>TSLFTTADHYHTPLGPDGTPHAFFEALRDEAETTPIGWSEAYGGHWVVAGYKEIQAVIQNTKAFSNKGVTFPRYETGEFELMMAGQDDPVHKKYRQLVAKPFSPEATDLFTEQLRQSTNDLIDARIELGEGDAATWLANEIPARLTAILLGLPPEDGDTYRRWVWAITHVENPEEGAEIFAELVAHARTLIAERRTNPGNDIMSRVIMSKIDGESLSEDDLIGFFTILLLGGIDNTARFLSSVFWRLAWDIELRRRLIAHPELIPNAV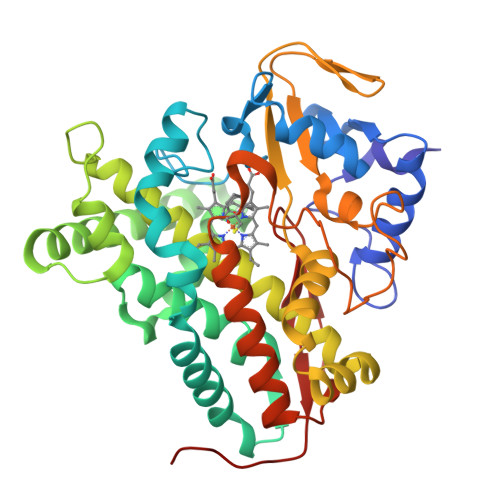DELLRFYGPAMVGRLVTQEVTVGDITMKPGQTAMLWFPIASRDRSAFDSPDNIVIERTPNRHLSLGHGIHRCLGAHLIRVEARVAITEFLKRIPEFSLDPNKECEWLMGQVAGMLHVPIIFPKGKRLSE[2x]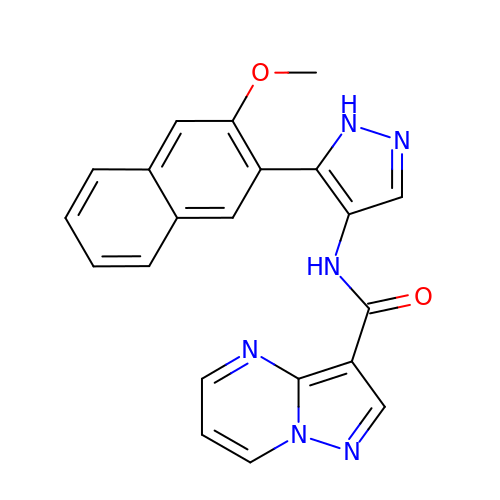N-[5-(3-methoxynaphthalen-2-yl)-1H-pyrazol-4-yl]pyrazolo[1,5-a]pyrimidine-3-carboxamide | C21 H16 N6 O2 | LGRPDWKAHUIEOE-UHFFFAOYSA-N>MFENVSTFEEAFNKLLKEVL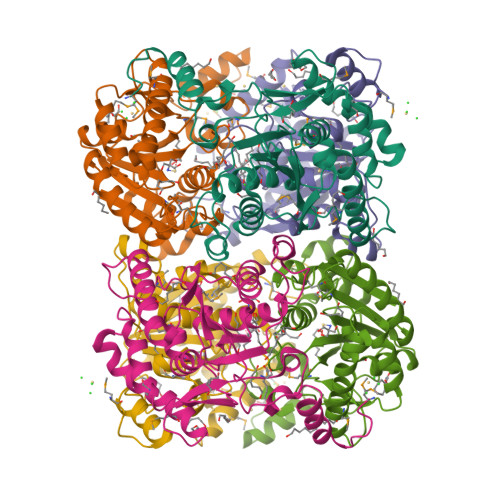EFNLENPFEDAKKVICIEPHPDDCAIGMGGTIKKLSDEGVEVIYICMTDGYMGTTDEKLSGHELALIRRREEEESAKLLGVRKIYWLNYRDTELPYSREVRKDLVKIIRKEKPDGVFAPDPWLPYESHPDHRRTGFLAIESVAFSQLPNFSNIDIDIGLKPHSVSFIALYYTHKPNYIVDITDLMELKLKAIRAHRSQFTDDIWETWEPFLRTVTMFYGEKIGVRYGEGFRVMPGLFYHITPFADLI[6x]> MGNTSIQTQSYRAVDKDAGQSRSYIIPFALLCSLFFLWAVANNLNDILLPQFQQAFTLTNFQAGLIQSAFYFGYFIIPIPAGILMKKLSYKAGIITGLFLYALGAALFWPAAEIMNYTLFLVGLFIIAAGLGCLETAANPFVTVLGPESSGHFRLNLAQTFNSFGAIIAVVFGQSLILSNVPHQSQDVLDKMSPEQLSAYKHSLVLSVQTPYMIIVAIVLLVALLIMLTKFPALQSDNHSDAKQGSFSASLSRLARIRHWRWAVLAQFCYVGAQTACWSYLIRYAVEEIPGMTAGFAANYLTGTMVCFFIGRFTGTWLISRFAPHKVLAAYALIAMALCLISAFAGGHVGLIALTLCSAFMSI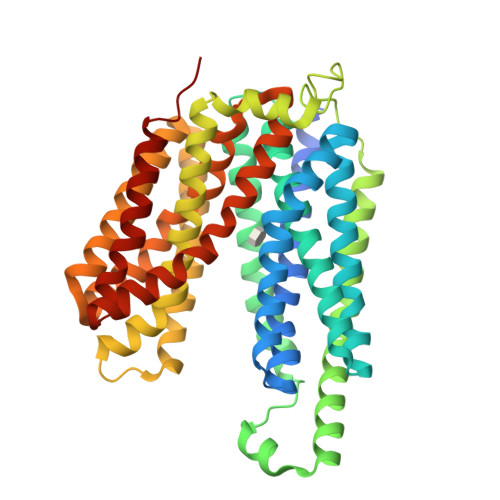QYPTIFSLGIKNLGQDTKYGSSFIVMTIIGGGIVTPVMGFVSDAAGNIPTAELIPALCFAVIFIFARFRSQTATN2-{2-[(1S,2S)-2-{[1-(8-methylquinolin-2-yl)piperidine-4-carbonyl]amino}cyclopentyl]ethyl}benzoic acid | C30 H35 N3 O3 | 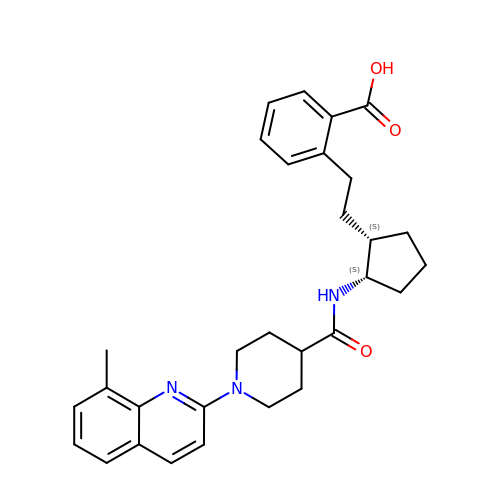NLKZRAQTODORFW-NVQXNPDNSA-N> MVAKGRIIRVTGPLVVADGMKGAKMYEVVRVGELGLIGEIIRLEGDKAVIQVYEETAGVRPGEPVVGTGASLSVELGPRLLTSIYDGIQRPLEVIREKTGDFIARGVTAPALPRDKKWHFIPKAKVGDKVVGGDIIGEVPETSIIVHKIMVPPGIEGEIVEIAEEGDYTIEEVIAKVKTPSGEIKELKMYQRWPVRVKRPYKEKLPPEVPLITGQRVIDTFFPQAKGGTAAIPGPFGSAKTVTQHQLAKWSDAQVVIYIGCGERGNEMTDVLEEFPKLKDPKTGKPLMERTVLIANTSNMPVAAREASIYTGITIAEYFRDMGYDVALMADSTSRWAEALREISGRLEEMPGEEGYPAYLASKLAEFYERAGRVVTLGSDYRVGSVSVIGAVSPPGGDFSEPVVQNTLRVVKVFWALDADL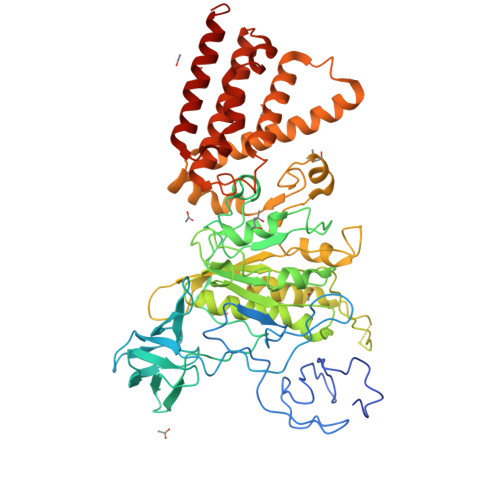ARRRHFPAINWLTSYSLYVDAVKDWWHKNIDPEWKAMRDKAMALLQKESELQEIVRIVGPDALPERERAILLVARMLREDYLQQDAFDEVDTYCPPEKQVTMMRVLLNFYDKTMEAINRGVPLEEIAKLPVREEIGRMKFERDVSKIRSLIDKTNEQFEELFKKYGA>[8x]MSNRDLFAELSSALVEAKQH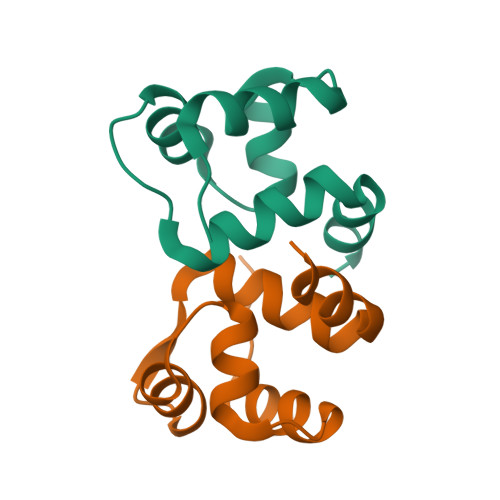SEGKLTLKTHHVNDVGELNISPDEIVSIREQFNMSRGVFARLLHTSSRTLENWEQGRSVPNGQAVTLLKLVQRHPETLSHIAEL>GAATLATLPAPINQIFPDADLAEGIRAVLQKASVTDVVTQEELESITKLVVAGEKVASIQGIEYLTNLEYLNLNGNQITDISPLSNLVKLTNLYIGTNKITDISALQNLTNLRELYLNEDNISDISPLANLTKMYSLNLGANHNLSDLSPLSNMTGLNYLTVTESKVKDVTPIANLT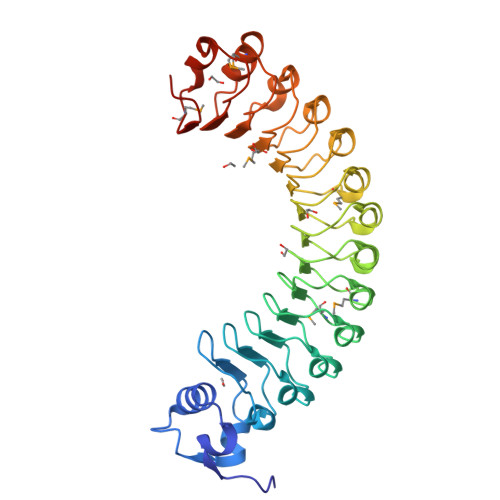DLYSLSLNYNQIEDISPLASLTSLHYFTAYVNQITDITPVANMTRLNSLKIGNNKITDLSPLANLSQLTWLEIGTNQISDINAVKDLTKLKMLNVGSNQISDISVLNNLSQLNSLFLNNNQLGNEDMEVIGGLTNLTTLFLSQNHITDIRPLASLSKMDSADFANQVIKK[2x]The self-labeling protein tags (SLPs) HaloTag7, SNAP-tag, and CLIP-tag allow the covalent labeling of fusion proteins with synthetic molecules for applications in bioimaging and biotechnology. The three most popular SLPs are HaloTag7 (HT7),14 SNAP-tag (SNAP),15 and CLIP-tag (CLIP)16. To guide the selection of an SLP–substrate pair and provide guidelines for the design of substrates, we report a systematic and comparative study of the labeling kinetics and substrate specificities of HaloTag7, SNAP-tag, and CLIP-tag. We complement these kinetic studies by reporting crystal structures of HT7 and SNAP covalently labeled with rhodamine-based fluorophores, providing a detailed understanding of their substrate preferences.

The HT7 variant HOB (halo-based oligonucleotide binder)52 features several positively charged surface mutations close to the substrate binding site, which were introduced to increase the labeling rates with chloroalkanes attached to oligonucleotides. Indeed, HOB shows a 3.13 ± 0.01-fold increase in kapp compared to that of HT7 with CA-Alexa488, while a decrease in kapp was observed with CA-TMR (2.09 ± 0.01-fold). This suggests that kinetics of negatively charged substrates might suffer from charge repulsions at the HT7 surface. HOB comprises four surface mutations compared to HT7 close to the substrate entry channel but opposite the TMR binding site. These mutations lead to a small but significant increase in labeling rates (3.1-fold) with negatively charged CA substrates relative to HT7. Only minor differences can be observed between the crystal structures of HOB and HT7 labeled with CA-TMR. Because the HOB mutations replace mostly negatively with positively charged residues, we analyzed the electrostatic potential of both proteins. While HT7 features an overall negatively charged surface around the substrate entry channel, HOB shows a positively charged patch opposite the fluorophore binding site. Hence, a putative electrostatic steering effect could explain the altered substrate preference of HOB despite the fact that its positive charges are on the opposite side of the fluorophore binding site.

> GIGTGFPFDPHYVEVLGERMHYVDVGPRDGTPVLFLHGNPTSSYVWRNIIPHVAPTHRCIAPDLIGMGKSDKPDLGYFFDDHVRFMDAFIEALGLEEVVLVIHDWGSALGFHWAKRNPERVKGIAFMEFIRPIPTWDEWPKFARKTFQAFRTKKVGRKLIIDQNVFIEGTLPMGVVRPLTEVEMDHYREPFLNPVDREPLWRFPNELPIAGEPANIVALVEEYMDWLHQSPVPKLLFWGTPGVLIPPAEAARLAKSLPNCKAVDIGPGLNLLQEDNPDLIGSEIARWLSTLEISG> GVVDSCCRNSCSFSTLRAYCDS;> NSLRACGPALMDMLRVAC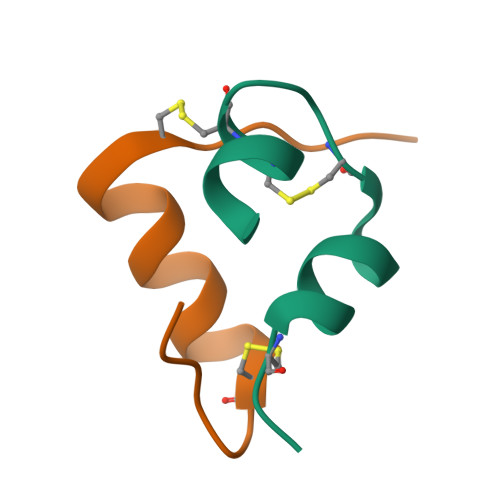PNGFNS>MVLIFHGKPVHGAIFDMDGTMFDTERLRFQTLQQASQELIGQEFSHEYLMQCLGLSATTAEKLAQRLYGVDVPYKEIRKRADEMELEHIRKHGVPIKKGLVQVLERLRKSGLRMAVATSSRRAIAEEYLINANVYKFFDVITCGDEVEQGKPHPEIFLKAASQLHLDANQCLMFEDSENGLTSAHTSKGLTILLKDIKEPNDEMLEKAHFYYDQMYDFLTDLDQFIPVMDMPEMQEPFPQSLNQLTVGIHGFGAIGGGYIAQILSHWDGYTKPKRIIASTRNSLFREAVNAFGTYSIRYGQFSYDERIENMSIVDSDNEQQMLEMYTHSSLIALCLPEQAIESESKIIAKGLYARFNSQLETCIEPLTFLIILNKVGAKYLVMKHLKEALLELTNDEDVTEHILKEHYFCDTVVNRMVSKLSNQNLYRQLRIKHNFLEQHLEDVEQEDQIEIEDCNKLTPDQLNQASIYVDNMRRNFQPGHILQSMDLILFHSETDMPIYVEKGSPLLEKLR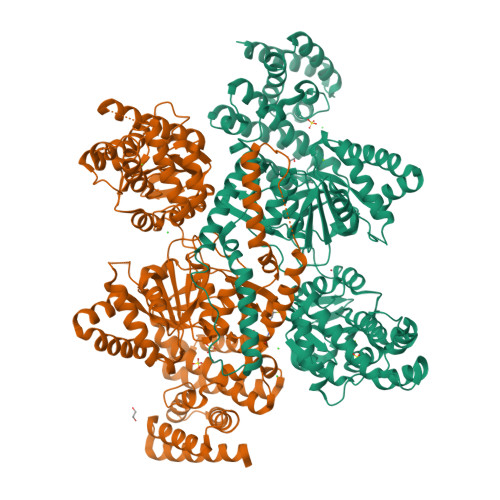QVVLVDQITDIQLIKNRLWNGVHAMLAWYASLMGYESIGVAMGDHLVKAFAENLIAEVKQGLAIVLPNYAKDLDRMSQSFLDSCEYAFKDPCQRVARDPLRKLNHNERVMASIAVNIRHDLPYKNLLKGAALGYAYAIQFLEIEETKAVEHLQQQIQNLDLSTAQRRQLEAELVQLIQYLFSEQGKQPLDIKSNNTKTTSTQYVAAALEHHHHHH[2x]6,6'-{[(2S)-3-aminopropane-1,2-diyl]bis(oxymethanediyl)}bis(4-methylpyridin-2-amine) 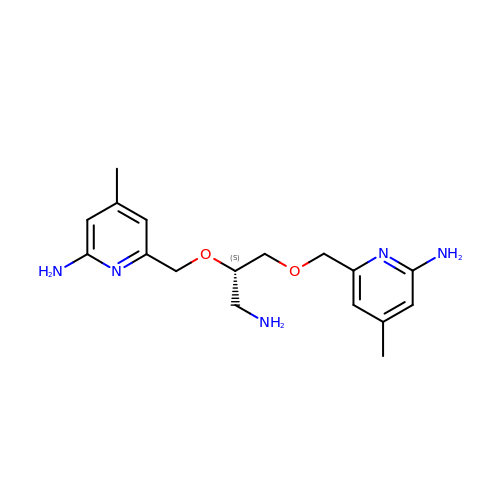| C17 H25 N5 O2 | FVCUZJIKIIWHJD-HNNXBMFYSA-N> MDFQNFVATLESFKDLKSGISGSRIKKLTTYALDHIDIESKIISLIIDYSRLCPDSHKLGSLYIIDSIGRAYLDETRSNSNSSSNKPGTCAHAINTLGEVIQELLSDAI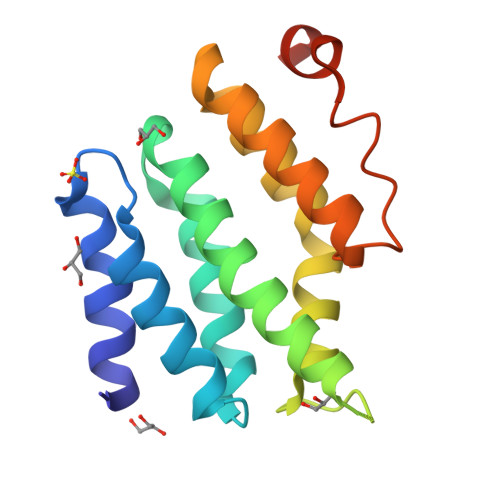AKSNQDHKEKIRMLLDIWDRSGLFQKSYLNAIRSKCFAAALEHHHHHH>MSNVPHKSSLPEGIRPGTVLRIRGLVPPNASRFHVNLLCGEEQGSDAALHFNPRLDTSEVVFNSKEQGSW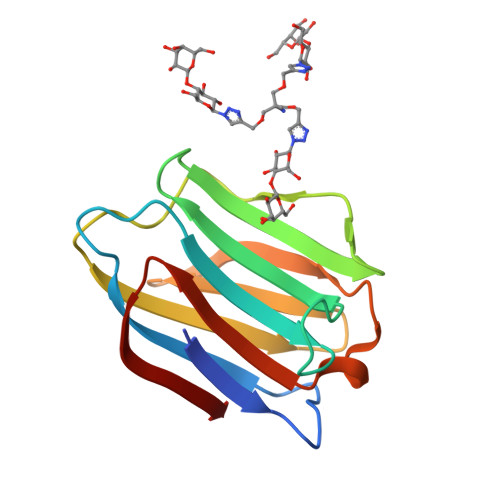GREERGPGVPFQRGQPFEVLIIASDDGFKAVVGDAQYHHFRHRLPLARVRLVEVGGDVQLDSVRIF[6x]(S)-2-({5-[4-(2-Amino-4-oxo-4,7-dihydro-3H-pyrrolo[2,3-d]-pyrimidin-6-yl)butyl]thiophene-3-carbonyl}amino)pentanedioic acid | C20 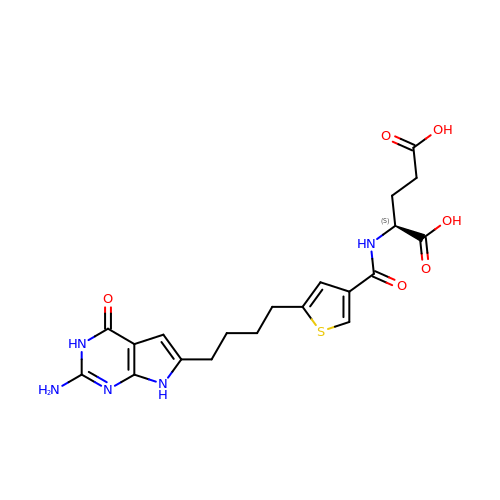H23 N5 O6 S | JBVKQLSCSCXKDY-AWEZNQCLSA-N> MGRGKVKPNRKSTGDNSNVVTMIRAGSYPKVNPTPTWVRAIPFEVSVQSGIAFKVPVGSLFSANFRTDSFTSVTVMSVRA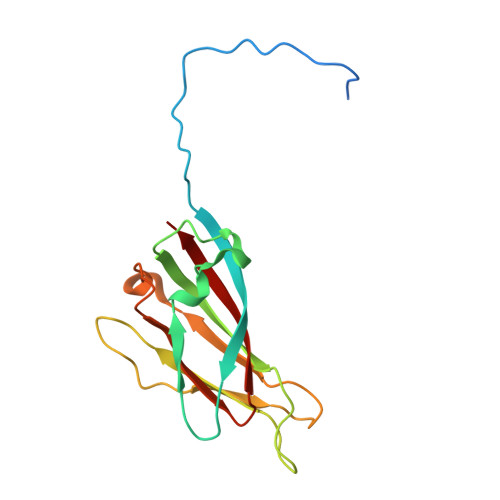WTQLTPPVNEYSFVRLKPLFKTGDSTEEFEGRASNINTRASVGYRIPTNLRQNTVAVDNVCEVRSNCRQVALVISCCFN>GVLAPVVPGKALEFPQDFGAHNDFRIEWWYVTGWLETPTGKPLGFQITFFRTATEIDRDNPSHFAPDQLIIAHVALSDPAIGKLQHDQKIARAGFDLAYARTGNTDVKLDDWIFVRETDGRYRTRIEAEDFTLTFILTPSQPLMLQGENGFSRKGPGAPQASYYYSEPHLQVSGIINRQGEDIPVTGTAWLDREWSSEYLDPNAAGWDWISANLDDGSALMAFQIRGKDDSKIWAYAALRDASGHTRLFTPDQVSFHPIRTWRSARTQAVYPVATRVLTGETEWQITPLMDDQELDSRASAGAVYWEGAVTFTRDGQPAGRGYME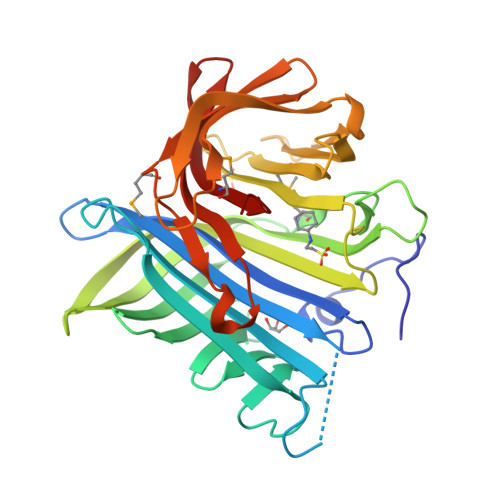LTGYVRPLSM[2x]>SNAMANIEIRQETPTAFYIKVHDTDNVAIIVNDNGLKAGTRFPDGLELIEHIPQGHKVALLDIPANGEIIRYGEVIGYAVRAIPRGSWIDESMVVLPEAPPLHTLPLATKVPEPLPPLEGYTFEGYRNADGSVGTKNLLGITTSVHCVAGVVDYVVKIIERDLLPKYPNVDGVVGLNHLYGCGVAINAPAAVVPIRTIHNISLNPNFGGEVMVIGLGCEKLQPERLLTGTDDVQAIPVESASIVSLQ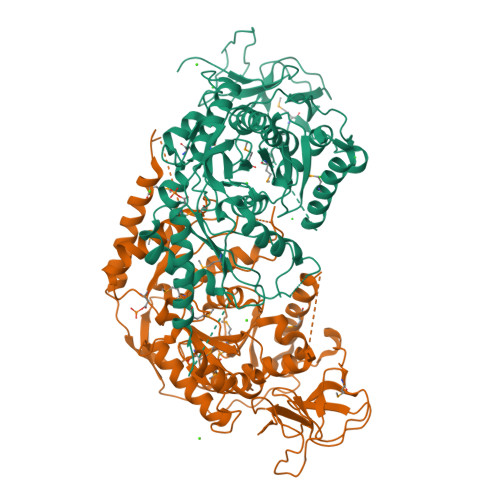DEKHVGFQSMVEDILQIAERHLQKLNQRQRETCPASELVVGMQCGGSDAFSGVTANPAVGYASDLLVRCGATVMFSEVTEVRDAIHLLTPRAVNEEVGKRLLEEMEWYDNYLNMGKTDRSANPSPGNKKGGLANVVEKALGSIAKSGKSAIVEVLSPGQRPTKRGLIYAATPASDFVCGTQQVASGITVQVFTTGRGTPYGLMAVPVIKMATRTELANRWFDLMDINAGTIATGEETIEEVGWKLFHFILDVASGKKKTFSDQWGLHNQLAVFNPAPVT[4x]>[4x]AECSVDIQGNDQMQFNTNAITVDKSCKQFTVNLSHPGNLPKNVMGHNWVLSTAADMQGVVTDGMASGLDKDYLKPDDSRVIAHTKLIGSGEK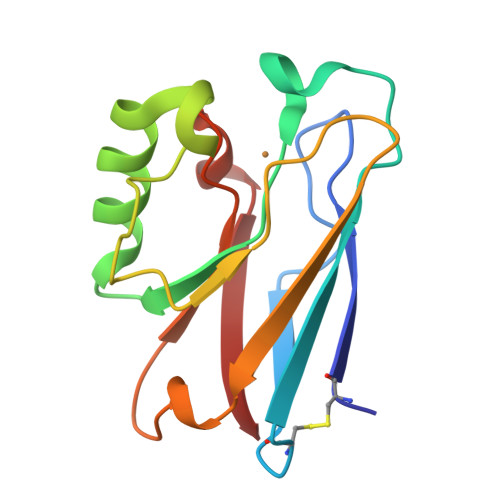DSVTFDVSKLKEGEQYMFFCAAAAHAAAMKGTLTLK> LKLCSPEEFTRLCREKTQEIYPIKEANGRTRKALIICNTEFKHLSLRYGANFDIIGMKGLLEDLGYDVVVKEELTAEGMESEMKDFAALSEHQTSDSTFLVLMSHGTLHGICGTMHSEKTP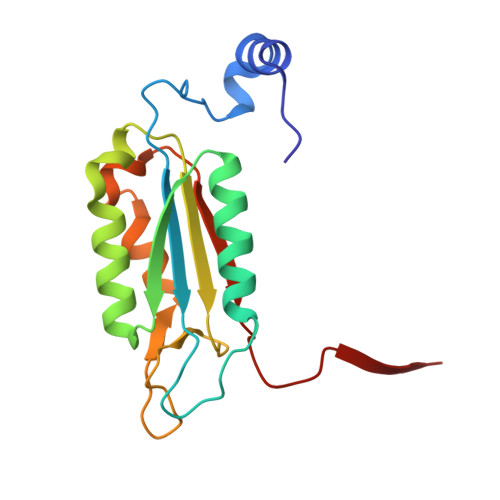DVLQYDTIYQIFNNCHCPGLRDKPKVIIVQAARGGNSGEMWIR> MILFDKNKRILKKYAKMVSKINQIESDLRSKKNSELIRLSMVLKEKVNSFEDADEHLFEAFALVREAARRTLGMRPFDVQVMGGIALHEGKVAEMKTGEGKTLAATMPIYLNALIGKGVHLVTVNDYLARRDALWMGPVYLFLGLRVGVINSLGKSYEVVWKNPDLARKAIEENWSVWPDGFNGEVLKEESMNKEAVEAFQVELKEITRKEAYLCDVTYGTNNEFGFDYLRDNLVLDYNDKVQRGHFYAIVDEADSVLIDEARTPLIISGPSKESPSVYRRFAQIAKKFVKDKDFTVDEKARTIILTEEGVAKAEKIIGVENLYDPGNVSLLYHLINALK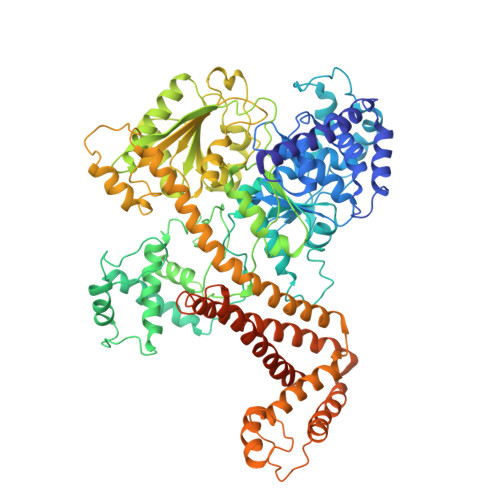ALHLFKKDVDYVVMNGEVIIVDEFTGRLLPGRRYSGGLHQAIEAKEGVPIKEESITYATITFQNYFRMYEKLAGMTGTAKTEESEFVQVYGMEVVVIPTHKPMIRKDHDDLVFRTQKEKYEKIVEEIEKRYKKGQPVLVGTTSIEKSELLSSMLKKKGIPHQVLNAKYHEKEAEIVAKAGQKGMVTIATNMAGRGTDIKLGPGVAELGGLCIIGTERHESRRIDNQLRGRAGRQGDPGESIFFLSLEDDLLRIFGSEQIGKVMNILKIEEGQPIQHPMLSKLIENIQKKVEGINFSIRKTLMEMDDVLDKQRRAVYSLRDQILLEKDYDEYLKDIFEDVVSTRVEEFCSGKNWDIESLKNSLSFFPAGLFDLDEKQFSSSEELHDYLFNRLWEEYQRKKQEIGEDYRKVIRFLMLRIIDDHWRRYLEEVEHVKEAVQLRSYGQKDPIVEFKKETYYMFDEMMRRINDTIANYVLRVVKVSEKDEKEAKEELGKIRLVHEEFNLVNRAMRRATEKKKKKDGLHSFGRIRVKR Streptococcus pneumoniae scavenges essential zinc ions from the host during colonization and infection. This is achieved by the ATP-binding cassette transporter, AdcCB, and two solute-binding proteins (SBPs), AdcA and AdcAII. AdcAII belongs to the cluster A-I subgroup of SBPs, consisting of a conserved structural fold of two (β/α)4 domains connected by a rigid α-helix, with the metal-binding site located at the interface between the N- and C-terminal lobes (Loisel et al., 2008; Yukl, 2017).

In this study, we investigated the Zn(II)-binding mechanism of AdcAII by mutating each of the four Zn(II)-coordinating residues in the SBP. Structural analyses of Zn(II)-bound AdcAII variants revealed that specific regions within the protein underwent conformational changes via direct coupling to each of the metal-binding residues. The binding site mutations impacted protein conformation and interaction with Zn(II) to differing extents. Quantitative in vitro metal-binding assays combined with affinity determination and phenotypic growth assays revealed that each of the four Zn(II)-coordinating residues contributes to metal binding by AdcAII. Intriguingly, the phenotypic growth impact of the mutant adcAII alleles was, in general, independent of affinity, suggesting that the Zn(II)-bound conformation of the SBP is crucial for efficacious metal uptake. Taken together, these data demonstrate the importance of SBP-metal complex conformation for bacterial Zn(II) uptake.

> HMGTGSLGGGFPGKGMKIVTSFYPIYAMVKEVSGDLNDVRMIQSSSGIHSFEPSANDIAAIYDADVFVYHSHTLESWAGSLDPNLKKSKVKVLEASEGMTLERVPGLEDVEAGDGVDEKTLYDPHTWLDPEKAGEEAQIIADKLSEVDSEHKETYQKNAQAFIKKAQELTKKFQPKFEKATQKTFVTQLTAFSYLAKRFGLNQLGIAGISPEQEPSPRQLTEIQEFVKTYKVKTIFTESNASSKVAETLVKSTGVGLKTLNPLESDPQNDKTYLENLEENMSILAEELKGNLYFQ>[2x]AQYEDGKQYTTLEKPVAGAPQVLEFFSFFCPHCYQFEEVLHISDNVKKKLPEGVKMTAYHVNFMGGDLGKDLTQAWAVAMALGVEDKVTVPLFEGVQKTQTIRSASDIRDVFINAGIKGEEYDAAWNSFVVKSLVAQQEKAAADVQLRGVPAMFVNGKYQLNPQGMDTSNMDVFVQQYADTVKYLSEKK

DsbA from E. coli K−12 (EcDsbA) was the first and is probably the best-characterised DSB enzyme to date. This 21 kDa periplasmic protein is a dithiol oxidase that catalyses disulphide bond formation between consecutive cysteines of unfolded polypeptides as they are translocated to the periplasm. EcDsbA consists of a canonical TRX domain, a hallmark of proteins involved in redox homeostasis, with an inserted helical domain. The TRX domain harbours the conserved active site CXXC (C30-P31-H32-C33 in EcDsbA) that is featured in many proteins of the TRX superfamily. The acidity of this groove originates from a cluster of negatively charged residues (E24, E37, E38, D44, E85, D86 and E94) that map along a buried channel in the interface between the TRX and helical domains of EcDsbA.

DsbA K58A and double-mutant E24A/K58A were crystalised in space group C2, with two molecules per asymmetric unit. The crystal structures of the three mutants containing the K58A mutation showed that the shorter alanine side chain at position 58 significantly expanded the size of the entrance to the buried channel. In all three crystal structures, a glycerol molecule, used for cryoprotection, was modelled into the electron density. The binding of glycerol displaced w2 in all three structures and hindered precise analysis of the water network in these mutants. However, examination of the three lysine mutant structures showed that w1 was strictly conserved, forming hydrogen bonds to the backbone amide of C33. When E37 was present in the protein structures, water w3 was observed to form a hydrogen bond with E37 in both K58A and E24A/K58A structures. Additional water molecules (labelled as w’ in Figure 4F–H) were modelled into the electron density in the buried channel in all the lysine mutants. E24A caused a 2.9-fold reduction in the initial rate, while K58A resulted in a 1.9-fold reduction in the initial rate. The K58A mutant exhibited an oxidation rate of 2.10 ± 0.17 × 106 M−1 s −1, which is also not statistically different from the wildtype. However, the double-mutant E24A/K58A yielded a rate constant of 1.47 ± 0.06 × 106 M−1 s −1, 35% slower than that of wildtype EcDsbA. These results indicated that E24A and K58A did influence DsbA oxidase activity, but its individual effect may be too small to be detected in this assay.>[22x]EEDLTEVKKDALENLRVYLCEKIIAERHFDHLRAKKILSREDTEEISCRTSSRKRAGKLLDYLQENPKGLDTLVESIRREKTQNFLIQKITDEVLK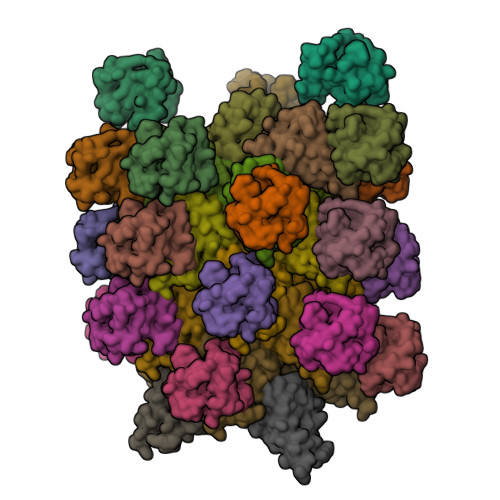LRNIKLEHLK;>[22x]TLNRLREPLLRRLSELLDQAPEGRGWRRLAELAGSRGRLRLSCLDLEQCSLKVLEPEGSPSLCLLKLMGEKGCTVTELSDFLQAMEHTEVLQLL>[2x]GDVAYELPAHTTRAQLSIDLVNNGDVEQQEKINSMRFIVFGSTPGGVRLDVNEHILLSTPETATDIDAQLLEVTSSNDILVVVIANEPQSLTSQLDGIANLLTLQEMIYDISSILNSDGQIISATG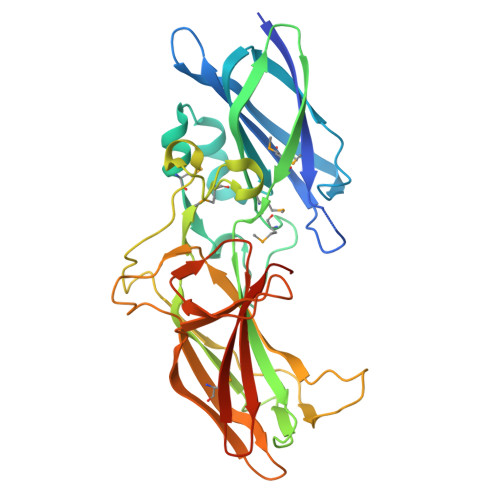MPMTGVIRDISIAPDETKTVQMVIERAVARVDVFIEAIDGGAVTGYTAGSTSVTLHNFSHDSYFVMGNVGNGTRDNADSSKNYGKVKEDVSESNLLTHSWTAATTETWAYSSAPGAENRKLLCSFYTAERLFKSDYSDRLSISMANVLKGPSDVTGITGKVIESVTKVDGTGSPTAQPFTEIRRNNVYQVTARVGKIGIQILTISVEDWGERQDIDLDMDL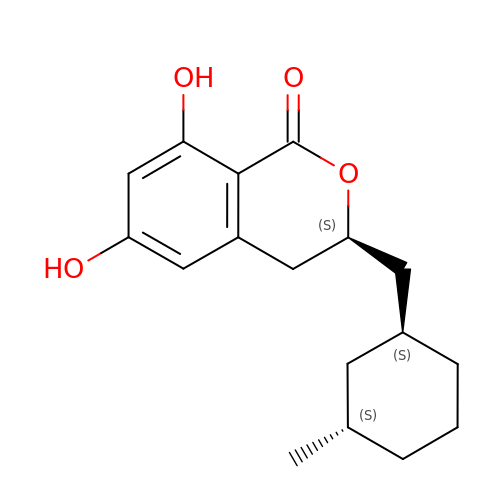(3~{S})-3-[[(1~{S},3~{S})-3-methylcyclohexyl]methyl]-6,8-bis(oxidanyl)-3,4-dihydroisochromen-1-one | C17 H22 O4 | ZGIJWPKFHHUCIH-MJVIPROJSA-N> GAMGSFNSIDVEINMYPVNKTSCNSSIGSSSTISTSELTITLTHEDCTPVFIGDYYSVVDKLATSGFFTNDKVHQDLTTQCKINLEIKCNSGRESRQLTPTTKVYLMPHSETVTVVGDCLSNLDVYIVYANTDAIYSDMDVVA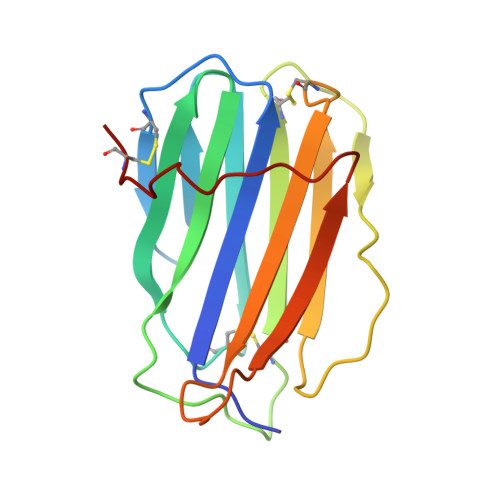YHTSYILNVDHIPPNDCERD5-methoxy-6-pyridin-4-yl-1~{H}-indole | C14 H12 N2 O | 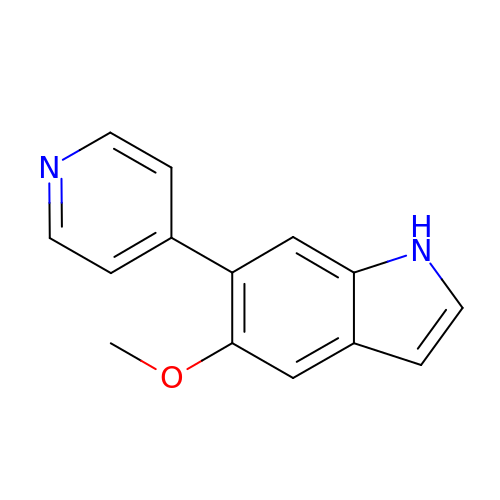CCGSQZWVGGCGET-UHFFFAOYSA-N> SGQNNVVGVHYKVGRRIGEGSFGVIFEGTNLLNNQQVAIKFEPRRSDAPQLRDEYRTYKLLAGCTGIPNVYYFGQEGLHNVLVIDLLGPSLEDLLDLCGRKFSVKTVAMAAKQMLARVQSIHEKSLVYRDIKPDNFLIGRPNSKNANMIYVVDFGMVKFYRDPVTKQHIPYREKKNLSGTARYMSINTHLGREQSRRDDLEALGHVFMYFLRGSLPWQGLKAATNKQKYERIGEKKQSTPLRELCAGFPEEFYKY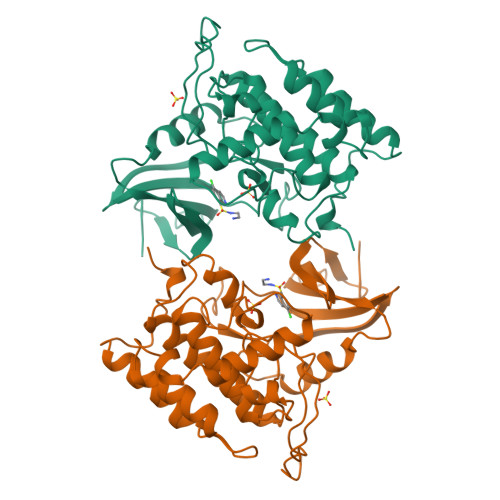MHYARNLAFDATPDYDYLQGLFSKVLERLNTTEDENFDWNLL> GSMSISISYSTTYSGWTVADYLADWSAYFGDVNHRPGQGVDGSNTGGFNPGPFDGSQYALQSTASDAAFIAGGDLHYTLFSNPSHTLWGKLDSIALGDTLTGGASSGGYALDSQEVSFSNLGLDSPIAQGRDGTVHKVVYGLMSGDSSALQGQIDALLKAVDP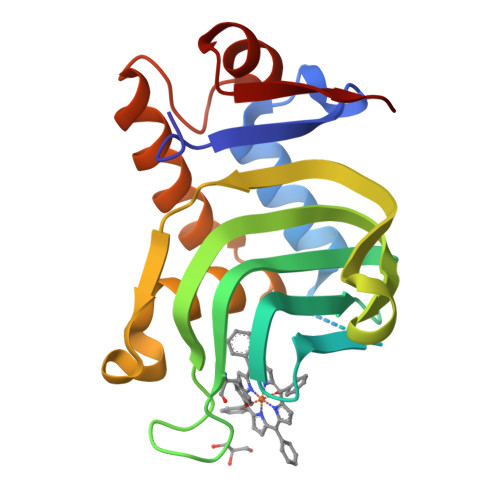SLSINSTFDQLAAAGVAHATPA> GIHHVSIKDVLSKYVQLLPNGSSEFRVVKEKDGSSEILTENQVTFDTKTTSEGLVEVTAKFSPNYSLEDGARYVLKFTVTSSQEALDAIAGDKKLEAGDAEGSDVNKLYSNKGASVTYSYGIGNSQTKTKEYSDNPTFKPSDPLTVPVEVEWQGVTGARTVITADQPSNVELKLVQKNKNGGSDNQDYRKTNVNVSKNVSNETRNFEKVAKGYQYDLIAPDVPAFTKEIKNVGTESNPSFKVIYKQLPSLTIKKVLEAENNLNKEFRIKVKLTSPDSKPLNGTFGEITVVNGEAEIRVEKRKRWRGILSYLP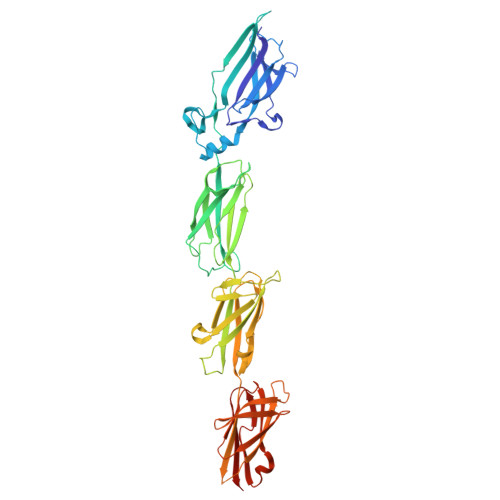RGTHYKVEEEAASTNGYHVTYENQEGDLNKDETSTVTNHKLPSLSVTKKVTGVFANLLKSFKITINIRDAQNSPLNGTYTATVNNKRTPLQFTNGRASIDLNKDQTIKIDGLPLDSHYTVEEETNSSRGYQVSYENQEGKLDGDKSATVTNNKNSVPET> MLKRSK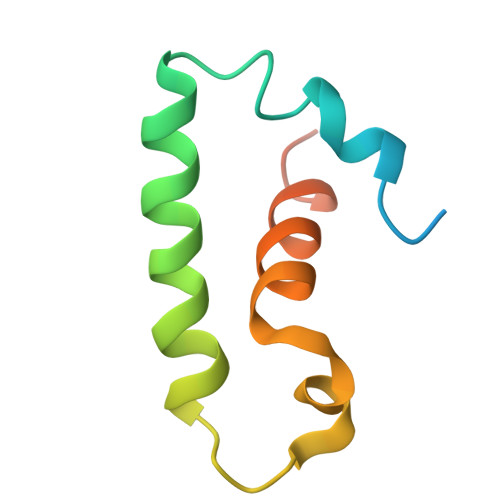FETTQSQIMHRAEDLISAASNRYRITVQVANRAKRRRYEEFESAEDAMMKPVLRAIIEMSDELTQPEIIGEI> ASAKELACQEITVPLCKGIGYQYTYM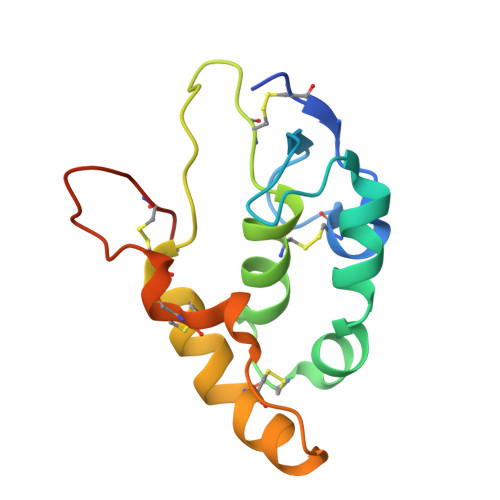PNQFNHDTQDEAGLEVHQFWPLVEIQCSPDLKFFLCSMYTPICLEDYKKPLPPCRSVCERAKAGCAPLMRQYGFAWPDRMRCDRLPEQGNPDTLCMDHHHHHH>MGAALGTGTRLAPWPGRACGALPRWTPTAPAQGCHSKPGPARPVPLKKRGYDVTRNPHLNKGMAFTLEERLQLGIHGLIPPCFLSQDVQLLRIMRYYERQQSDLDKYIILMTLQDRNEKLFYRVLTSDVEKFMPIVYTPTVGLACQHYGLTFRRPRGLFITIHDKGHLATMLNSWPEDNIKAVVVTDGERILGLGDLGCYG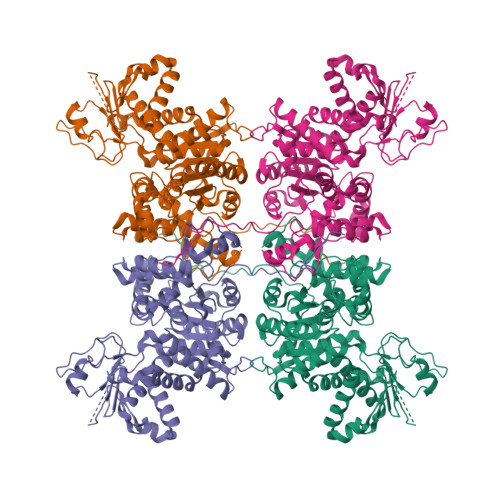MGIPVGKLALYTACGGVNPQQCLPVLLDVGTNNEELLRDPLYIGLKHQRVHGKAYDDLLDEFMQAVTDKFGINCLIQFEDFANANAFRLLNKYRNKYCMFNDDIQGTASVAVAGILAALRITKNKLSNHVFVFQGAGEAAMGIAHLLVMALEKEGVPKAEATRKIWMVDSKGLIVKGRSHLNHEKEMFAQDHPEVNSLEEVVRLVKPTAIIGVAAIAGAFTEQILRDMASFHERPIIFALSNPTSKAECTAEKCYRVTEGRGIFASGSPFKSVTLEDGKTFIPGQGNNAYVFPGVALGVIAGGIRHIPDEIFLLTAEQIAQEVSEQHLSQGRLYPPLSTIRDVSLRIAIKVLDYAYKHNLASYYPEPKDKEAFVRSLVYTPDYDSFTLDSYTWPKEAMNVQTV[4x]>[2x]MFPGSVIRKLS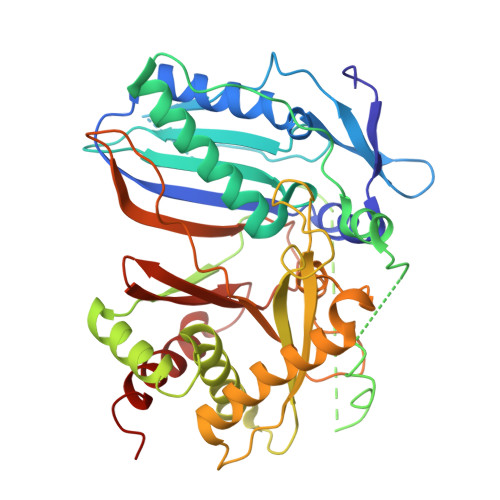HSEEVFAQYEVFTSMTIQLRGVIDVDALSDAFDALLETHPVLASHLEQSSDGGWNLVADDLLHSGICVIDGTAATNGSPSGNAELRLDQSVSLLHLQLILREGGAELTLYLHHCMADGHHGAVLVDELFSRYTDAVTTGDPGPITPQPTPLSMEAVLAQRGIRKQGLSGAERFMSVMYAYEIPATETPAVLAHPGLPQAVPVTRLWLSKQQTSDLMAFGREHRLSLNAVVAAAILLTEWQLRNTPHVPIPYVYPVDLRFVLAPPVAPTEATNLLGAASYLAEIGPNTDIVDLASDIVATLRADLANGVIQQSGLHFGTAFEGTPPGLPPLVFCTDATSFPTMRTPPGLEIEDIKGQFYCSISVPLDLYSCAVYAGQLIIEHHGHIAEPGKSLEAIRSLLCTVPSEYGWIME GPR34 is a recently identified G-protein coupled receptor, which has an immunomodulatory role and recognizes lysophosphatidylserine (LysoPS) as a putative ligand. Here, we report two cryo-electron microscopy (cryo-EM) structures of human GPR34-Gi complex bound to an sn-3 LysoPS derivative and the potent M1 agonist. GPR34 adopts the canonical GPCR topology of a heptahelical transmembrane bundle (7TM), with an extracellular N-terminus, three extracellular loops (ECLs), three intracellular loops (ICLs), and a short amphipathic helix 8 (H8) oriented parallel to the membrane. The ligand-binding pocket of GPR34 extends from the centre of ECL2 to the middle of TM4–5, forming an ~25-Å cleft that is laterally open toward the membrane.

S3E-LysoPS is an analogue of sn-3-type 18:1 LysoPS, with an ethoxy group at the sn-1 position. Local refinement with the mask of the receptor improved local resolution of the extracellular half of the receptor, and the resulting cryo-EM maps allowed modelling of the entire complexes, including agonists. S3E-LysoPS fits into this cleft, oblique to the receptor. The head group and the acyl chain of S3E-LysoPS fit within the hydrophilic and hydrophobic pockets, respectively. The head group of S3E-LysoPS fits into the pocket, with a U-shaped conformation. The phosphate group engages in electrostatic interactions with the positively charged residues, R1102.60, R208ECL2, and K210ECL2, but does not form direct interactions, such as hydrogen bonds. Moreover, the carboxylate of the serine moiety forms a direct salt bridge with R2866.55 and hydrogen bonds with Y1353.33 and N3097.35. The amine group forms an electrostatic interaction with E3107.36 and a hydrogen bond with the backbone carbonyl group of F205ECL2. The acyl chain of S3E-LysoPS is bent at the cis-9 double bond and fits along the L-shaped pocket. Moreover, R2866.55A mutation abolishes agonist response, whereas alanine mutations of R208ECL2, N3097.35, and E3107.36 reduced potency by ~10–30-fold.

> DYKDDDDAMGRSHTITMTTTSVSSWPYSSHRMRFITNHSDQPPQNFSATPNVTTCPMDEKLLSTVLTTSYSVIFIVGLVGNIIALYVFLGIHRKRNSIQIYLLNVAIADLLLIFCLPFRIMYHINQNKWTLGVILCKVVGTLFYMNMYISIILLGFISLDRYIKINRSIQQRKAITTKQSIYVCCIVWMLALGGFLTMIILTLKKGGHNSTMCFHYRDKHNAKGEAIFNFILVVMFWLIFLLIILSYIKIGKNLLRISKRRSKFPNSGKYATTARNSFIVLIIFTICFVPYHAFRFIYISSQLNVSSCYWKEIVHKTNEIMLVLSSFNSCLDPVMYFLMSSNIRKIMCQLLFRRFQGEPSRSESTSEFKPGYSLHDTSVAVKIQSSSKSTENLYFQ>[6x]VEYKNTICPPRQDYRYWYFVAELTIGVNYDINSTIIGECHMSESYIDRNANIVLTGYGLKINMT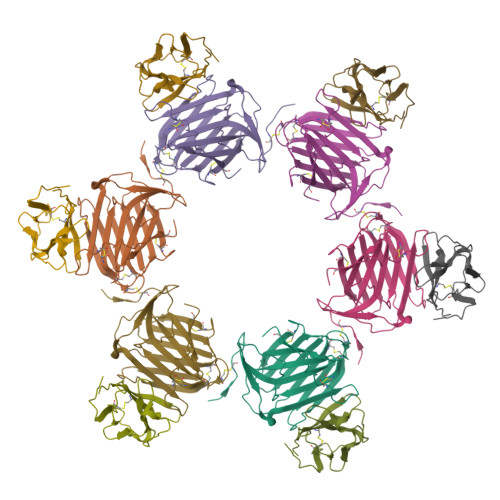IMDTDQRFVAAAEGVGKDNKLSVLLFTTQRLDKVHHNISVTITCMEMNCGTTKYNSDLPESIHKSSSCDITINGSCVTCVNLETDPTKINPHYLHPKNKYLYHNSEYSMRGSYGVTFIDELNQCLLDIKELSYDICYRE;>LKIQAYFNETADLPCQFANSQNQSLSELVVFWQDQENLVLNEVYLGKEKFDSVHSKYMGRTSFDSDSWTLRLHNLQIKDKGLYQCIIHHKKPTGMIRIHQMNSELSVLANFSQPEIVPISNITENVYINLTCSSIHGYPEPKKMSVLLRTKNSTIEYDGVMQKSQDNVTELYDVSISLSVSFPDVTSNMTIFCILETDKTRLLSSPFSIELED[6x]> MENPLQKARILVNQLEKYLDRYAKEYDVEHLAGPQGHLVMHLYKHPDKDMSIKDAEEILHISKSVASNLVKRMEKNGFIAIVPSKTDKRVKYLYLTHLGKQKATQFEIFL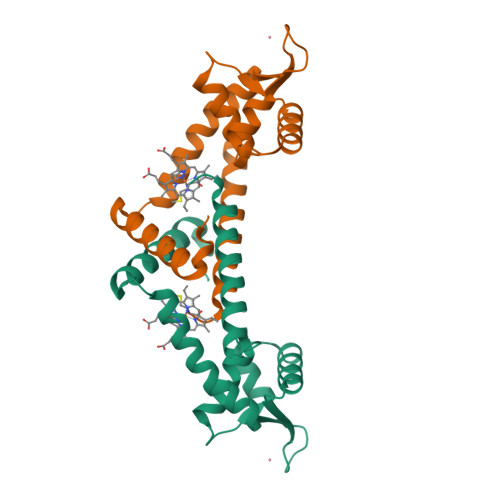EKLHSTMLAGITKEEIRTTKKVIRTLAKNMAMEDFDSLEVLFQ> GSHMASPNGQTKPLPALKLALEYIVPCMNKHGICVVDDFLGKETGQQIGDEVRALHDTGKFTDGQLVSQKSDSSKDIRGDKITWIEGKEPGCETIGLLMSSMDDLIRHCNGKLGSYKINGRTKAMVACYPGNGTGYVRHVDNPNGDGRCVTCIYYLNKDWDAKVSGGILRIFPEGKAQFADIEPKFDRLLFFWSDRHNPHEVQPAYA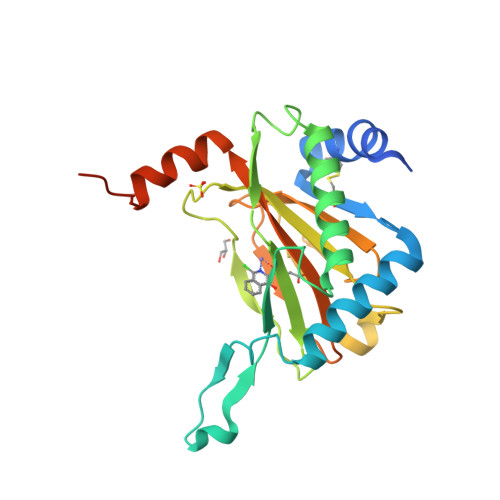TRYAITVWYFDADERARAKVKYLTGEKGVRVELNKPSDSVGKDVF>[2x]MEAAHSKSTEECLAYFGVSETTGLTPDQVKRHLEKYGHNELPAEEGKSLWELVIEQFEDLLVRILLLAACISFVLAWFEEGEETITAFVEPFVILLILIANAIVGVWQERNAENAIEALKEYEPEMGKVYRADRKSVQRIKARDIVPGDIVEVAVGDKVPADIRILSIKSTTLRVDQSILTGESVSVIKHTEPVPDPRAVNQDKKNMLFSGTNIAAGKALGIVATTGVSTEIGKIRDQMAATEQDKTPLQQKLDEFGEQLSKVISLICVAVWLINIGHFNDPVHGGSWIRGAIYYFKIAVALAVAAIPEGLPAVITTCLALGTRRMAKKNAIVRSLPSVETLGCTSVICSDKTGTLTTNQMSVCKMFIIDKVDGDFCSLNEFSITGSTYAPEGEVLKNDKPIRSGQFDGLVELATICALCNDSSLDFNETKGVYEKVGEATETALTTLVEKMNVFNTEVRNLSKVERANACNSVIRQLMKKEFTLEFSRDRKSMSVYCSPA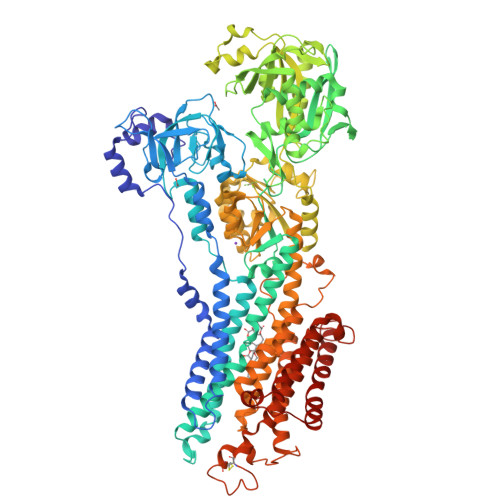KSSRAAVGNKMFVKGAPEGVIDRCNYVRVGTTRVPMTGPVKEKILSVIKEWGTGRDTLRCLALATRDTPPKREEMVLDDSSRFMEYETDLTFVGVVGMLDPPRKEVMGSIQLCRDAGIRVIMITGDNKGTAIAICRRIGIFGENEEVADRAYTGREFDDLPLAEQREACRRACCFARVEPSHKSKIVEYLQSYDEITAMTGDGVNDAPALKKAEIGIAMGSGTAVAKTASEMVLADDNFSTIVAAVEEGRAIYNNMKQFIRYLISSNVGEVVCIFLTAALGLPEALIPVQLLWVNLVTDGLPATALGFNPPDLDIMDRPPRSPKEPLISGWLFFRYMAIGGYVGAATVGAAAWWFMYAEDGPGVTYHQLTHFMQCTEDHPHFEGLDCEIFEAPEPMTMALSVLVTIEMCNALNSLSENQSLMRMPPWVNIWLLGSICLSMSLHFLILYVDPLPMIFKLKALDLTQWLMVLKISLPVIGLDEILKFIARNYLEG>[2x]MDHLKHLQQLQNIERIVLSGIVLANHKIEEVHSVLEPSDFYYPPNGLFFEIALKLHEEDCPIDENFIRQKMPKDKQIKEEDLVAIFAASPIDNIEA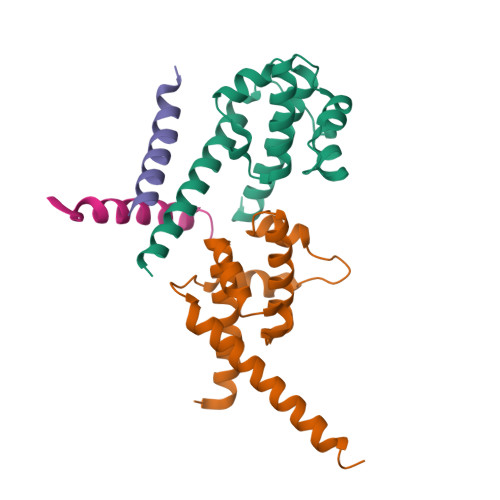YVEEIKNASIKRKLFGLANTIREQAHH;> IKNASIKRKLFGLANTIREQAL;> VEEIKNASIKRKLFGLANTIREQALE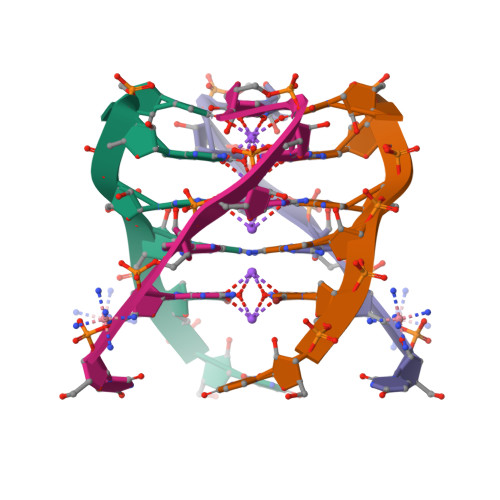> UGAGGU> MSLADHLTELRSRL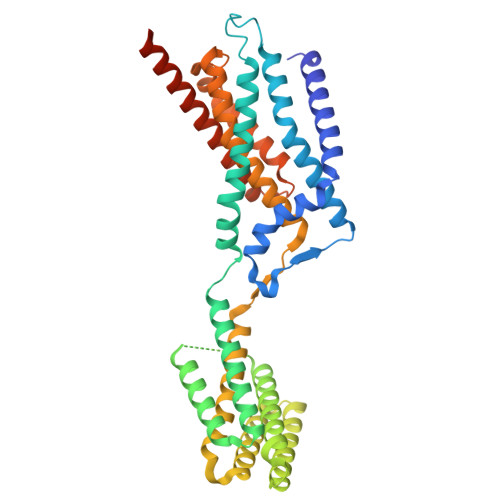MRATIAVLILGTISLVFAKPIFGLLMQPVLDALPPENRSLIYTSGIEELNVLMKVGVYAGIFLTTPVILMQIWGFVSPGLYPEERRFAAPFVAFGSIAFLLGAAFAYFAVLPSMFTFLLNEEETLALEQRLDTARLRADDALRFLRLGEAEEAGRIAKETSTQLRAEGQGQAPAPEVAPAASVEMTGRLDGLGRLLDAASVGYGAQSRGVLRQAVEKRVEAVTAYEKKDFAAAAAAMDGSASLLAGIAPTRTEELAGLWRLEKELATAHAAHEAARWTRPMLSMHEQLSLVLLLILAFGIIFELPLVMALLGVVGVVKSSWLFRYQRHAFVVALIAAAIITPTGDVVNLSLMAGPMLLAYELGVLLVWMVERRRARNSAETGITPASGSENLYFQ>[2x]SSRGHSTLPRTLMAPRM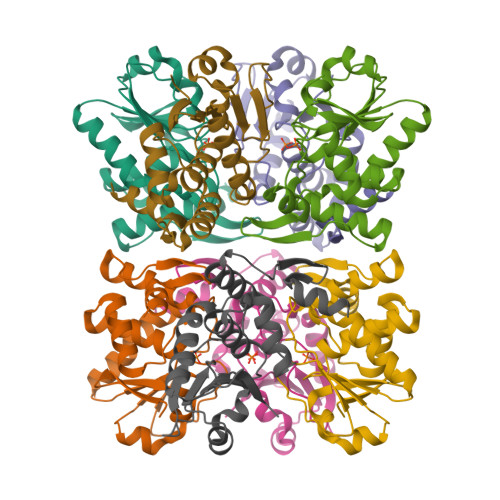ISEGDIGGIAQITSSLFLGRGSVASNRHLLQARGITCIVNATIEIPNFNWPQFEYVKVPLADMPHAPIGLYFDTVADKIHSVSRKHGATLVHCAAGVSRSATLCIAYLMKFHNVCLLEAYNWVKARRPVIRPNVGFWRQLIDYERQLFGKSTVKMVQTPYGIVPDVYEKESRH> MAIQNPYTAYQQNSVNTATPGELTLMLYNGC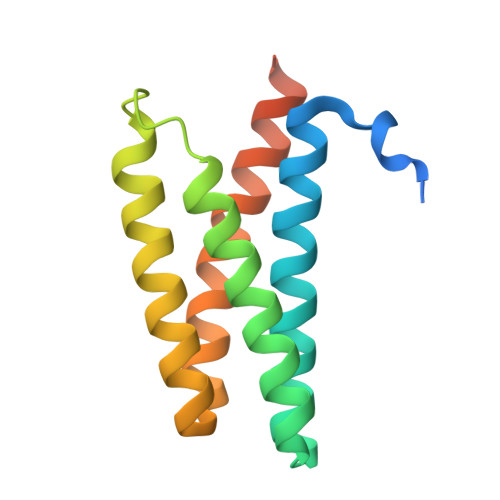LKFIRLAAQAIENDDMERKNENLIKAQNIIQELNFTLNRNIELSASMGAMYDYMYRRLVQANIKNDTGMLAEVEGYVTDFRDAWKQAIQSERKDRHGSGGIA> DKGKLSLQDVAELIRARACQRVVVMVGAGISTPSGIPDFRSPGSGLYSNLQQYDLPYPEAIFELPFFFHNPKPFFTLAKELYPGNYKPNVTHYFLRLLHDKGLLLRLYTQNIDGLERVSGIPASKLVEAHGTFASATCTVCQRPFPGEDIRADVMADRVPRCPVCTGVVKPDIVFFGEPLPQRFLLHVVDFPMADLLLILGTSLEVEPFASLTEAVRSSVPRLLINRDLVGPLAWHPRSRDVAQLGDVVHGVESLVELLGWTEEMRDLVQRETGKLDGPDK;> ATKAAR

Lysine lactylation (Kla) is a novel histone post-translational modification discovered in late 2019. Emerging biological and structural evidence suggests that Sirtuins are not limited to erasing acetyl groups from lysine residues but can also remove other forms of acyl groups. The zinc-binding domain and Rossmann fold domain make up the highly conserved catalytic core of Sirtuins. Our findings indicate that SIRT3 exhibits higher delactylation activity compared to other human Sirtuins, especially on H4K16 site.

Among the tested combination of Sirtuins and lactyl peptides, SIRT3 showed a higher delactylation activity on H4K16la and H3K23la peptide. Crystals of H3K23la(L)-SIRT3 and H4K16la(L)-SIRT3 complexes diffracted to 2.0 Å and 2.5 Å resolution, respectively. Each structure contains 1 SIRT3 molecule, 1 zinc atom, and 1 lactyl peptide in each asymmetric unit. The catalytic pocket of SIRT3 displayed half-hydrophobic and half-hydrophilic characters. In both structures, F180, I230, I291, and V292 of SIRT3 formed a preconfigured hydrophobic cage that accommodated the hydrocarbon portion of the lactyl group. While in the SIRT3-H3K23la(L) structure, due to the crystallization conditions involving glycerol, two glycerol molecules’ hydroxyl groups replaced the water molecule’s position and contributed to the formation of the water bridge, resulting in a robust hydrogen bond system.>[2x]SNAMTDAAIAEKDLGNAAYKQKDFEKAHVHYDKAIELDPSNITFYNNKAAVYFEEKKFAECVQFCEKAVEVGRETRADYKLIAKAMSRAGNAFQKQNDLSLA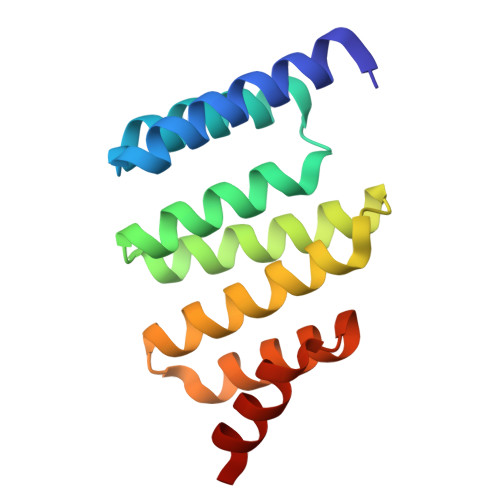VQWFHRSLSEFRDPELVKKVKELEK> AIGEFMVSLPRMVYPQPKVLTPCRKDVLVVTPWLAPIVWEGTFNIDILNEQFRLQNTTIGLTVFAIKKYVAFLKLFLETAEK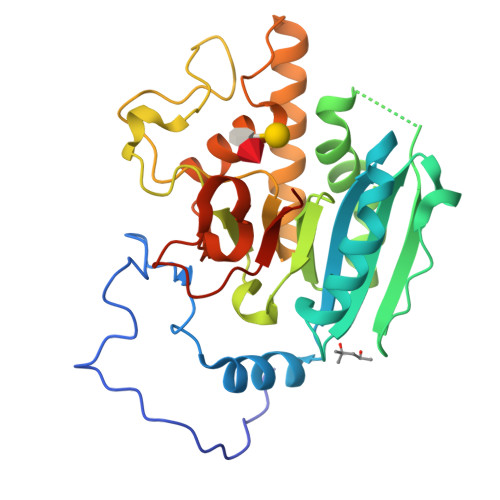HFMVGHRVHYYVFTDQPAAVPRVTLGTGRQLSVLEVGAYKRWQDVSMRRMEMISDFCERRFLSEVDYLVCVDVDMEFRDHVGVEILTPLFGTLHPSFYGSSREAFTYERRPQSQAYIPKDEGDFYYMGAFFGGSVQEVQRLTRACHQAMMVDQANGIEAVWHDESHLNKYLLRHKPTKVLSPEYLWDQQLLGWPAVLRKLRFTAVPKNHQAVRNP>[2x]AMGAPKPPQEPDMNNLPENPIPQHQAKFVLNTIKAVKRNREAVPFLHPVDTVKLNVPFYYNYIPRPMDLSTIERKINLKAYEDVSQVVDDFNLMVKNCKKFNGEAAGISKMATNIQAQFEKLMVKVPPKELPAGTNVA

BET proteins are chromatin-associated factors that regulate transcription and chromatin remodelling. BET proteins bind chromatin through their two BDs (BD1 and BD2), which specifically recognize histones acetylated on lysine residues. The BDs from C. albicans Bdf1 (CaBdf1) share 31–46% sequence identity with human BET BDs and 58–66% identity with those from ScBdf1 and hence are likely to bind multi-acetylated H3 and H4 tails. In conclusion, Bdf1 BDs are required for the viability and virulence of C. albicans and can be selectively targeted by small-molecule inhibitors without compromising human BET BD function.

The most active compound was dibenzothiazepinone 3, an analogue of 1 in which the cyclopropyl, oxadiazole and pyrazine groups are replaced by smaller methyl, carboxyamidyl and tetrahydrofuran groups, respectively. HTRF and ITC assays showed that 3 inhibits CaBdf1 BD1 with low-micromolar affinity and three- to fivefold selectivity relative to human Brd4 BD1. The crystal structure of CaBdf1 BD1 bound to 3 shows that the compound is slightly rotated within the binding pocket compared to 1. Consequently, in a structural alignment with Brd4 BD1, the steric hindrance observed for 1 due to the larger Trp81 and Leu94 side chains is largely relieved for compound 3, explaining the reduced selectivity of this compound. (Both enantiomers of 3 are equally active, consistent with the lack of interaction between the BD and the tetrahydrofuran ring). Liquid culture assays show that 3 has little effect on the growth of C. albicans strains expressing either WT Bdf1 or Bdf1 inactivated in BD1, but significantly inhibited the growth of strains inactivated in BD2, consistent with the specificity of compound 3 for BD1. A dose–response curve revealed a cellular EC50 value of 35±7 μM, corresponding to a 20-fold cell shift relative to the IC50 value determined by HTRF in vitro (or sevenfold relative to the Kd by ITC). At this concentration, compound 3 showed relatively little cytotoxicity towards mammalian cells (EC50 >100 μM). Our chemical screen identified a dibenzothiazepinone compound, 3, that selectively inhibited CaBdf1 BD1 and displayed antifungal activity against susceptible strains. Specifically, strains expressing Bdf1 mutants in which BD1 was the lone functional BD (mutants bdf1-bd2Δ and bdf1-Y425F) were sensitive to 3, consistent with this compound's selectivity for CaBdf1 BD1, whereas all other strains with a functional BD2 were insensitive, arguing strongly against a potential off-target effect.> SAEKLFTPLKVGAVTAPNRVFMAPLTRLRSIEPGDIPTPLMGEYYRQRASAGLIISEATQISAQAKGYAGAPGLHSPEQIAAWKKITAGVHAEDGRIAVQLWHTGRISHSSIQPGGQAPVSASALNANTRTSLRDENGNAIRVDTTTPRALELDEIPGIVNDFRQAVANAREAGFDLVELHSAHGYLLHQFLSPSSNQRTDQYGGSVENRARLV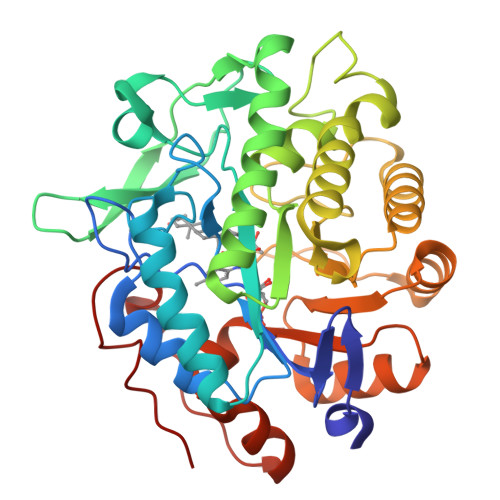LEVVDAVCNEWSADRIGIRVSPIGTFQNVDNGPNEEADALYLIEELAKRGIAYLHMSETDLAGGKPYSEAFRQKVRERFHGVIIGAGAYTAEKAEDLIGKGLIDAVAFGRDYIANPDLVARLQKKAELNPQRPESFYGGGAEGYTDYPSL> MRGSHHHHHHGSMPETNPNAPPRPDSLLNPSDALKHLEEYPRGDGLSLQELMDSRKNGGLTYNDFLVLPGHINFPASDVSLQSKATKNIVLNTPFLSSPMDTV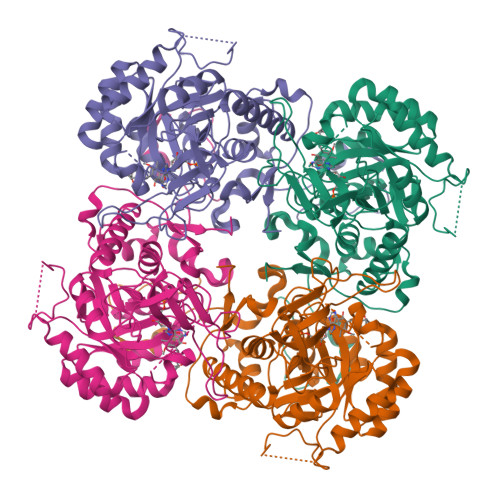TEDRMAIALALHGGLGIIHHNCSAEEQAAMVRRVKKYENGFITDPLCLGPDATVGDVLEIKAKFGFCGVPITETGEPDSKLLGIVTGRDVQFQDAETPIKSVMTTEVVTGSSPITLEKANSLLRETKKGKLPIVDSNGHLVSLVARSDLLKNQNYPYASKVPESKQLYCGAAIGTRPGDKDRLKLLAEAGLDVVVLDSSQGNSVYQIEFIKWIKQTYPKIDVIAGNVVTREQAAQLIAAGADGLRIGMGSGSICITQEVMAVGRPQGTAVYAVAEFASRFGIPCIADGGIGNIGHIAKALALGASAVMMGGLLAGTTESPGEYFYHEGKRVKVYRGMGSIEAMEHTQRGSASGKRSILGLDNAATARYFSEADAVKVAQGVSGDVADKGSINKFVPYLFTGLQHSLQDAAIKSVSELHSCARSGSLRFELRTASAQLEGGVHGLNSYTKRLFA;> MRGSHHHHHHGSMPETNPNAPPRPDSLLNPSDALKHLEEYPRGDGLSLQELMDSRKNGGLTYNDFLVLPGHINFPASDVSLQSKATKNIVLNTPFLSSPMDTVTEDRMAIALALHGGLGIIHHNCSAEEQAAMVRRVKKYENGFITDPLCLGPDATVGDVLEIKAKFGFCGVPITETGEPDSKLLGIVTGRDVQFQDAETPIKSVMTTEVVTGSSPITLEKANSLLRETKKGKLPIVDSNGHLVSLVARSDLLKNQNYPYASKVPESKQLYCGAAIGTRPGDKDRLKLLAEAGLDVVVLDSSQGNSVYQIEFIKWIKQTYPKIDVIAGNVVTREQAAQLIAAGADGLRIGMGSGSICITQEVMAVGRPQGTAVYAVAEFASRFGIPCIADGGIGNIGHIAKALALGASAVMMGGLLAGTTESPGEYFYHEGKRVKVYRGMGSIEAMEHTQRGSASGKRSILGLDNAATARYFSEADAVKVAQGVSGDVADKGSINKFVPYLFTGLQHSLQDAGIKSVSELHSCARSGSLRFELRTASAQLEGGVHGLNSYTKRLFA> MKCLVTGGNVKVLGKAVHSLSRIGDELYLEPLEDGLSLRTVNSSRSAYACFLFAPLFFQQYQAATPGQDLLRCKILMKSFLSVFRSLAMLEKTVEKCCISLNGRSSRLVVQLHCKFGVRKTHNLSFQDCESLQAVFDPASCPHMLRAPARVLGEAVLPFSPALAEVTLGIGRGRRVILRSYHEEEADSTAKAMVTEMCLGEEDFQQLQAQEGVAITFCLKEFRGLLSFAESANLNLSIHFDAPGRPAIFTIKDSLLDGHFVLATLSDTDS;> MHHHHHHKFRAKIVDGACLNHFTRISNMIAKLAKTCTLRISPDKLNFILCDKLANGGVSMWCELEQENFFNEFQMEGVSA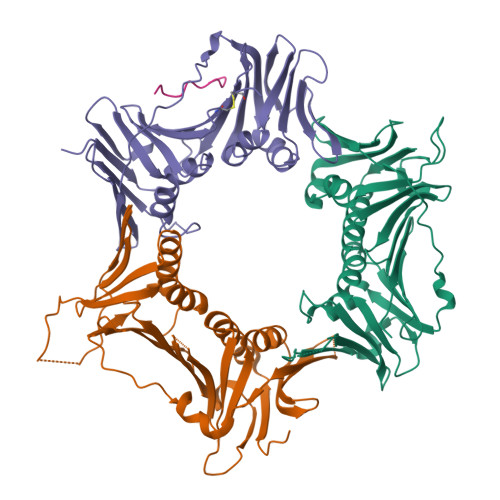ENNEIYLELTSENLSRALKTAQNARALKIKLTNKHFPCLTVSVELLSMSSSSRIVTHDIPIKVIPRKLWKDLQEPVVPDPDVSIYLPVLKTMKSVVEKMKNISNHLVIEANLDGELNLKIETELVCVTTHFKDLGNPPLASESTHEDRNVEHMAEVHIDIRKLLQFLAGQQVNPTKALCNIVNNKMVHFDLLHEDVSLQYFIPALS;> MPLLTQQIQDEDDQYSLVASLDNVRNLSTILKAIHFREHATCFATKNGIKVTVENAKCVQANAFIQAGIFQEFKVQEESVTFRINLTVLLDCLSIFGSSPMPGTLTALRMCYQGYGYPLMLFLEEGGVVTVCKINTQEPEETLDFDFCSTNVINKIILQSEGLREAFSELDMTSEVLQITMSPDKPYFRLSTFGNAGSSHLDYPKDSDLMEAFHCNQTQVNRYKISLLKPSTKALVLSCKVSIRTDNRGFLSLQYMIRNEDGQICFVEYYCCPDEEVPESES;> TDWVDPSFDDF>MGDTKEQRILRYVQQNAKPGDPQSVLEAIDTYCTQKEWAMNVGDAKGQIMDAVIREYSPSLVLELGAYCGYSAVRMARLLQPGARLLTMEINPDCAAITQQMLNFAGLQDKVTILNGASQDLIPQLKKKYDVDTLDMVFLDHWKDRYLPDTLLLEKCGLLRKGTVLLADNVIVPGTPDFLAYVRGSSSFECTHYSSY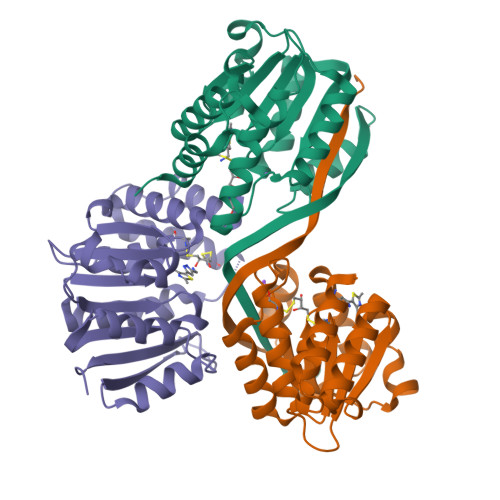LEYMKVVDGLEKAIYQGPSSPDKS[3x]> MDFDMIEEKKDSVIVRNVENFELKDIFDCGQCFRWHRQENGNY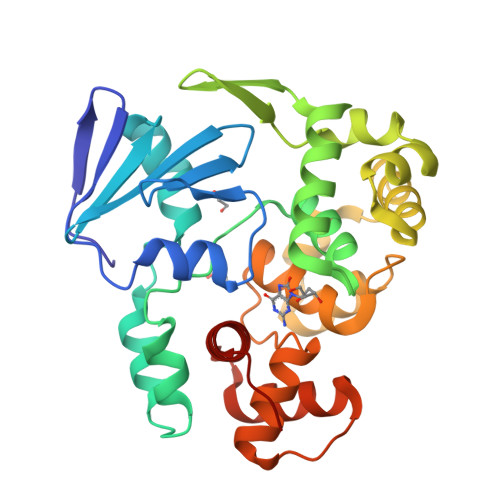IGIAFEKVVEVQKIGEDVVIYNINEEEFKNVWSEYFDLYRDYGEIKKELSRDPLLKKSVDFGEGIRILRQDPFEILLSFIISANNRIPMIKKCINNISEKAGKKLEYKGKIYYAFPTVDKLHEFTEKDFEECTAGFRAKYLKDTVDRIYNGELNLEYIKSLNDNECHEELKKFMGVGPQVADCIMLFSMQKYSAFPVDTWVKKAMMSLYVAPDVSLKKIRDFGREKFGSLSGFAQQYLFYYARENNIQL N-[(2S,3R,4E)-1,3-dihydroxyoctadec-4-en-2-yl]tetracosanamide | C42 H83 N 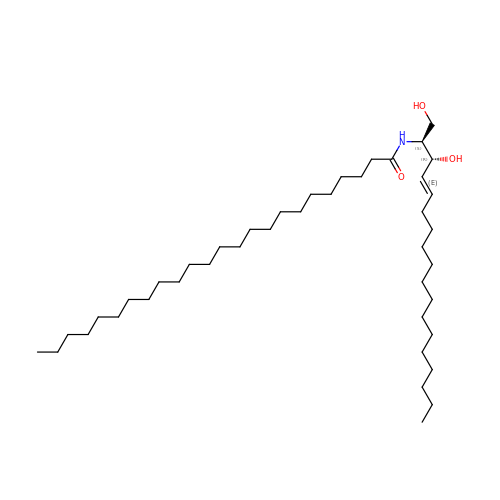O3 | ZJVVOYPTFQEGPH-AUTSUKAISA-N> GAMVPKTEDQRPQLDPYQILGPTSSRLANPGSGQIQLWQFLLELLSDSSNSSCITWEGTNGEFKMTDPDEVARRWGERKSKPNMNYDKLSRALRYYYDKNIM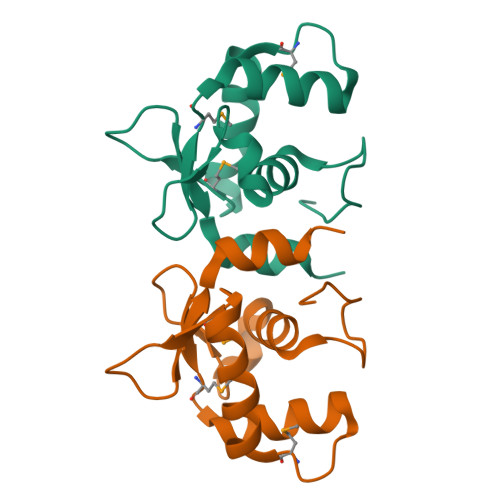TKVHGKRYAYKFDFHGIAQALQPHPPE>[2x]GSGAVSIASSKVSAQYTSTVPPSHYIETWAKTHPEWKAVEVATGFLGSQKIVTEDWTYKKLNETANQVANLIIHASLHGRAIAVSLDRSLIAFAIIVGIMKSGNTYVPIEAGLPNDRKSFLLRDSRAAMAFVCDNNFDGVELPPETKVLDTKNQSFIENLSTQDTSDILNNYPENLDAYLLYTSGSTGTPKGVR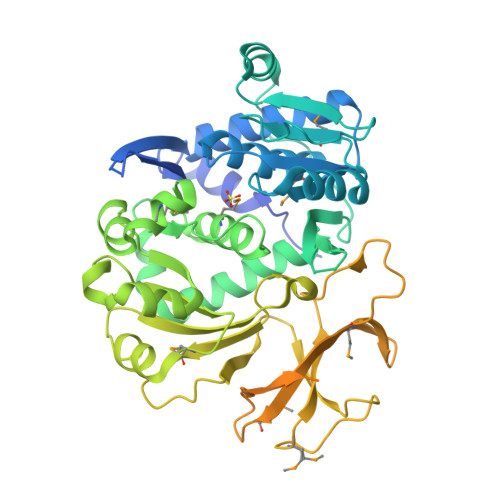VSRHNLSSFSDAWGKLIGNVAPKSLELGGVGKFLCLASRAFDVHIGEMFLAWRFGLCAVTGERLSMLDDLPRTFRELGVTHAGIVPSLLDQTGLVPEDAPHLVYLGVGGEKMTPRTQQIWSSSDRVALVNVYGPTEVTIGCSAGRILPDSDTRCIGHPLGDSVAHVLAPGSNEHVKKGMAGELVIEGSLVANGYLNRPDAKGFCDINGRKMYRTGDIVRMDADSSILFLGRKDEQVKVRGQRLELGEVSEVIRSLSPTDIDVVTLLLNHPGTSKQFLVSFVASSGAAVRGELRWINENYKEINNSLRQACEQTLPAYMVPDFIIPISFIPLRDTSAKTDAKALEHMFHTLSLGELFGESSSLVNKPTT> GVDYKYKQKPKYQVRWKIIESYEGNSYTFIDPTQLPYNEKWEFPRNNLQFGKTLGAGAFGKVVEATAFGLGKEDAVLKVAVKMLKSTAHADEKEALMSELKIMSHLGQHENIVNLLGACTHGGPVLVITEYCCYGDLLNFLRRKSRVLETDPAFAIANSTASTRDLLHFSSQVAQG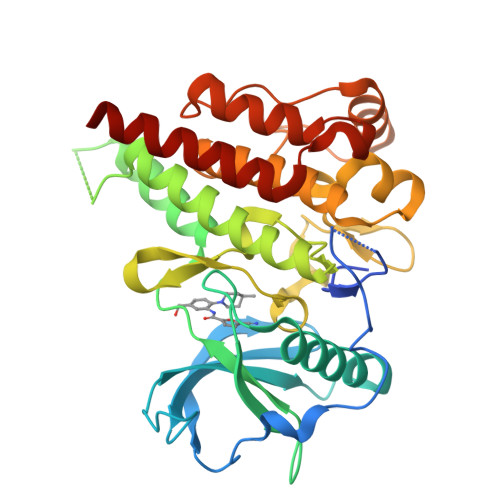MAFLASKNCIHRDVAARNVLLTNGHVAKIGDFGLARDIMNDSNYIVKGNARLPVKWMAPESIFDCVYTVQSDVWSYGILLWEIFSLGLNPYPGILVNSKFYKLVKDGYQMAQPAFAPKNIYSIMQACWALEPTHRPTFQQICSFLQEQAQEDRRERD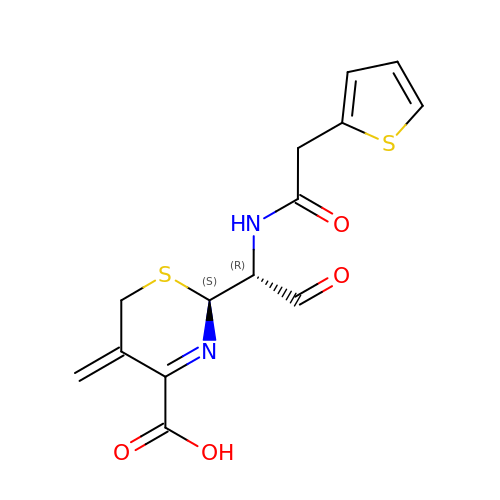(2S)-5-methylidene-2-{(1R)-2-oxo-1-[(thiophen-2-ylacetyl)amino]ethyl}-5,6-dihydro-2H-1,3-thiazine-4-carboxylic acid | C14 H14 N2 O4 S2 | FYGLCWWPHIWVKN-MFKMUULPSA-N As a type II transmembrane protein, comprising 274 amino acid residues, TMEM106B localizes to late endosomes and lysosomes. TMEM106B consists of an N-terminal cytosolic domain, a transmembrane helix, and a glycosylated C-terminal luminal domain (LD) that can be shed upon cleavage by lysosomal proteases. Here, we show that TMEM106B, a lysosomal transmembrane protein, can serve as an alternative receptor for SARS-CoV-2 entry into angiotensin-converting enzyme 2 (ACE2)-negative cells. Using X-ray crystallography, cryogenic electron microscopy (cryo-EM), and hydrogen-deuterium exchange mass spectrometry (HDX-MS), we show that the luminal domain (LD) of TMEM106B engages the receptor-binding motif of SARS-CoV-2 spike.

To enable biochemical and structural studies, we produced the luminal portion of human TMEM106B (residues 118–274, designated TMEM106BLD) by overexpression in human cells. The protein crystallized following partial deglycosylation by endoglycosidase H, and the structure was refined to 2.6 Å resolution. The final model spanning TMEM106B residues 118–261 revealed a compact fibronectin type III (Fn3) domain, an ubiquitous 7-bladed β sandwich fold, closely related to immunoglobulin domains. In TMEM106B, the domain is crowned by a short α helix (α1, residues 208–216), which is inserted into a loop between the canonical Fn3 β strands 5 and 6 and stabilized by a disulfide bond between Cys214 and Cys253. Endoglycosidase H cleaves N-linked glycans within the chitobiose core, leaving N-acetyl-D-glucosamine (NAG) attached to the protein. Concordantly, four NAG residues were found in the structure, linked to TMEM106B Asn residues 145, 151, 164, and 256. The N-terminal portion of the protein, not present in the crystallized construct, comprises a cytoplasmic tail (residues 1–96) and a single-pass transmembrane region (residues 97–117). To further confirm that the spike-TMEM106B interaction is required for SARS-CoV-2 infection, we used our structural data to identify six putative spike-binding residues in TMEM106B, mutated each residue to alanine, and tested whether these TMEM106B mutants still supported SARS-CoV-2 infection. Substitutions M210A and F213A had the most pronounced effect on virus infectivity.

> METDTLLLWVLLLWVPGSTGDAAQPRSIDVKYIGVKSAYVSYDVQKRTIYLNITNTLNITNNNYYSVEVENITAQVQFSKTVIGKARLNNITIIGPLDMKQIDYTVPTVIAEEMSYMYDFCTLISIKVHNIVLMMQVTVTTTYFGHSEQISQERYQYVDCGRNTTYQLGQSEYLNVLQPQQGSGENLYFQSAGHHHHHH>[2x]MADCCTPRKKLCWCVLLFFLVAGITGGAIGIYKWHYSGLNRWHGAGSTADFQKIIQERCDTYTQTIRPGSRSRNCQAIRQAFMSAFISKDPCKATKEDYNSLINLAPPTVPCGQQVFWSKTKELAHEYAKRRRLMTLEDTLLGYLADGLRWCGEPGSSDLNIWSCPDWRKDCRTNYLS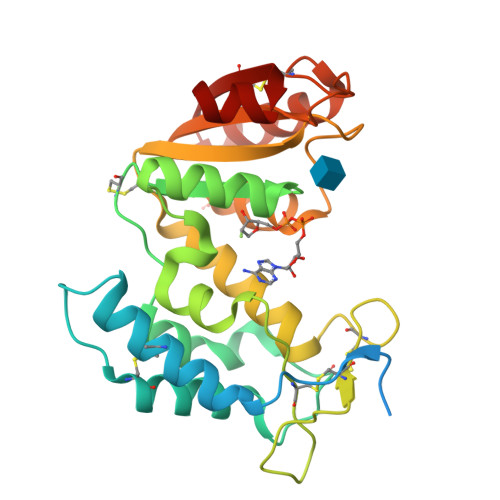VFWEVLSERFAESACNTVRVVLNGSLENAFDSMSIFGRVEAPNLRPQVELEAWLVHDTGKPPSDSCSGSSIRKLKSILDGRNVKFRCMDNLSRDQFLQRS> MAVKVEYDLKRLRNIGIAAHIDAGKTTTTERILYYTGRIHKIGEVHEGAATMDFMEQERERGITITAAVTTCFWKDHRINIIDTPGHVDFTIEVERSMRVLDGAIVVFDSSQGVEPQSETVWRQAEKYKVPRIAFANKMDKTGADLWLVIRTMQERLGARPVVMQLPIGREDTFSGIIDVLRMKAYTYGNDLGTDIREIPIPEEYLDQAREYHEKLVEVAADFDENIMLKYLEGEEPTEEELVAAIRKGTIDLKITPVFLGSALKNKGVQLLLDAVVDYLPSPLDIPPIKGTTPEGEVVEIHPDPNGPLAALAFKIMADPYVGRLTFIRVYSGTLTSGSYVYNTTKGRKERVARLLRMHANHREEVEELKAGDLGAVVGLKETITGDTLVGED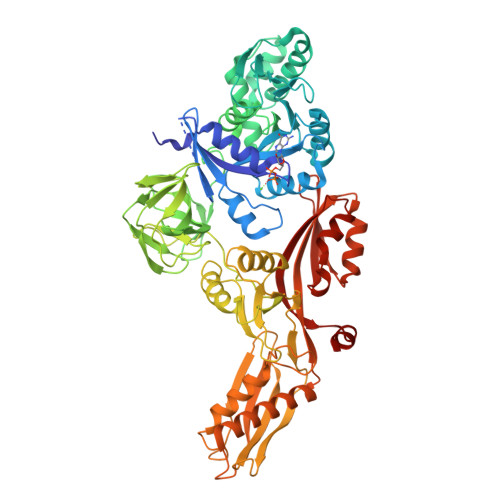APRVILESIEVPEPVIDVAIEPKTKADQEKLSQALARLAEEDPTFRVSTHPETGQTIISGMGELHLEIIVDRLKREFKVDANVGKPQVAYRETITKPVDVEGKFIRLTGGRGQYGHVKIKVEPLPRGSGFEFVNAIVGGVIPKEYIPAVQKGIEEAMQSGPLIGFPVVDIKVTLYDGSYHEVDSSEMAFKIAGSMAIKEAVQKGDPVILEPIMRVEVTTPEEYMGDVIGDLNARRGQILGMEPRGNAQVIRAFVPLAEMFGYATDLRSKTQGRGSFVMFFDHYQEVPKQVQEKLIKGQ> GQSNSNNWRWFDDRS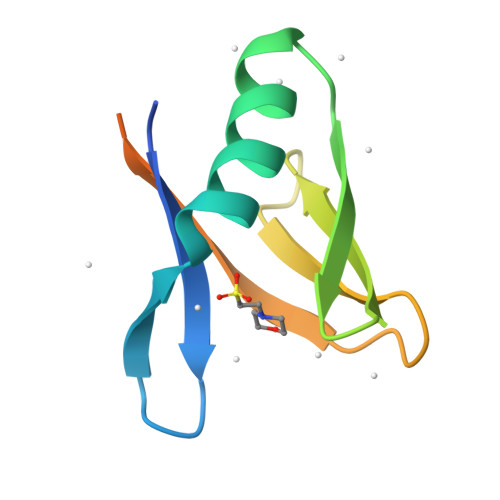GRWCSYSASNNSTIDSAWKSGETSVRFTAGRRRYTVQFTTMVQVNEETGNRRPVMLTLLRVPRLNKNSKNSNGQEL>[2x]GSMDNLLRHLKISKEQITPVVLVVGDPGRVDKIKVVCDSYVDLAYNREYKSVECHYKGQKFLCVSHGVGSA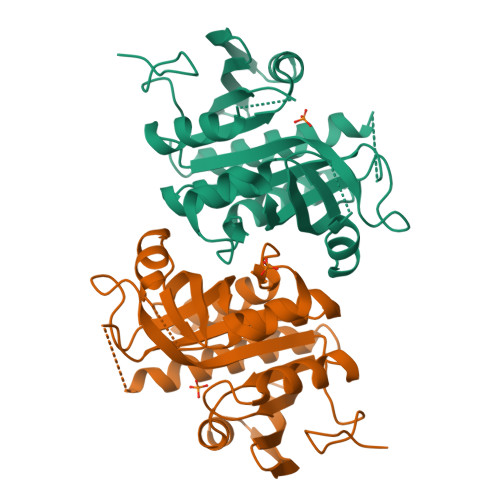GCAVCFEELCQNGAKVIIRAGSCGSLQPDLIKRGDICICNAAVREDRVSHLLIHGDFPAVGDFDVYDTLNKCAQELNVPVFNGISVSSDMYYPNKIIPSRLEDYSKANAAVVELELATLMVIGTLRKVKTGGILIVDGCPFKWDEGDFDNNLVPHQLENMIKIALGACAKLATKYA> ANPLYQKHIISINDLSRDDLNLVLATAAKLKANPQPELLKHKVIASCFFEASTRTRLSFETSMHRLGASVVGFSDSANTSLGKKGETLADTISVISTYVDAIVMRHPQEGAARLATEFSGNVPVLNAGDGSNQHPTQTLLDLFTIQETQGRLDNLHVAMVGDLKYGRTVHSLTQALAKFDGNRFYFIAPDALAMPQYILDMLDEKGIAWSLHSSIEEVMAEVDILYMTRVQKERL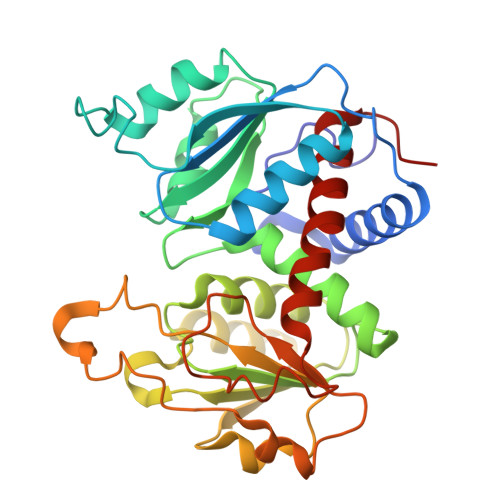DPSEYANVKAQFVLRASDLHNAKANMKVLHPLPRVDEIATDVDKTPHAWYFQQAGNGIFARQALLALVLNRDLVL>MEHKRGHVLAVPYPAQGHITPFRQFCKRLHFKGLKTTLALTTFVFNSINPDLSGPISIATISDGYDHGGFETADSIDDYLKDFKTSGSKTIADIIQKHQTSDNPITCIVYDAFLPWALDVAREFGLVATPFFTQPCAVNYVYYLSYINNGSLQLPIEELPFLELQDLPSFFSVSGSYPAYFEMVLQQFINFEKADFVLVNSFQELELHENELWSKACPVLTIGPTIPSIYLDQRIKSDTGYDLNLFESKDDSFCINWLDTRPQGSVVYVAFGSMAQLTNVQMEELASAVSNFSFLWVVRSSEEEKLPSGFLETVNKEKSLVLKWSPQLQVLSNKAIGCFLTHCGWNSTMEALTFGVPMVAMPQWTDQPMNAKYIQDVWKAGVRVKTEKESGIAKREEIEFSIKEVMEGERSKEMKKNVKKWRDLAVKSLN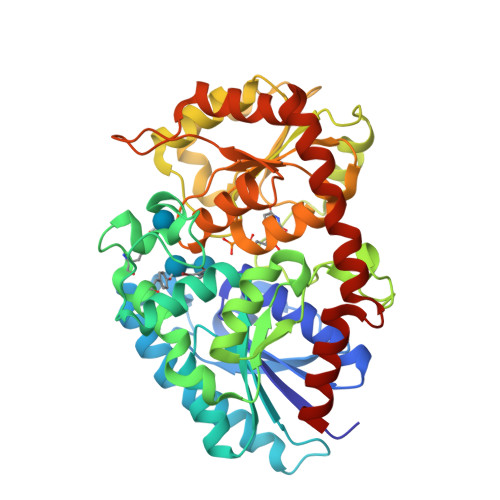EGGSTDTNIDTFVSRVQSK[2x]> HYRKTGSLLPTLPKLP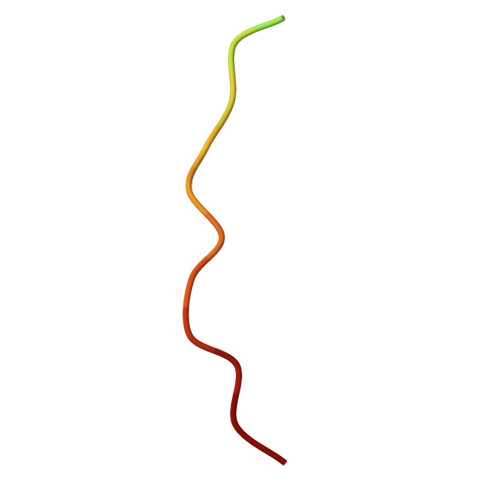SLS> MILDADYITEDGKPVIRVFKKEKGEFKIDYDRDFEPYIYALLKDDSAIEDIKKITAERHGTTVRVTRAERVKKKFLGRPVEVWKLYFTHPQDVPAIRDKIREHPAVVDIYEYDIPFAKRYLIDRGLIPMEGDEELRMLAFDIETLAHAGAAAGAGPILMISYADEEGARVITWKNIDLPYVESVSTEKEMIKRFLKVIQEKDPDVLITYNGDNFDFAYLKKRSEMLGVKFILGRDGSEPKIQRMGDRFAVEVKGRIHFDLYPVIRRTINL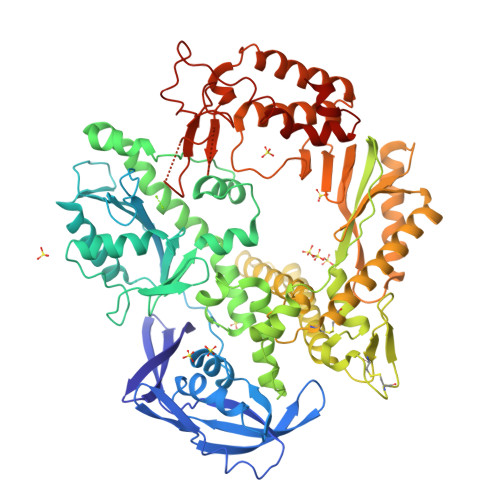PTYTLETVYEPVFGQPAEKVYAEEIAEAWASGEGLERVARYSMEDAKATYELGKEFFPMEAQLSRLVGQSLWDVSRSSTGNLVEWFLLRKAYERNDVAPNKPDERELARRTESYAGGYVKEPEKGLWENIVYLDYKSLYPSIIITHNVSPDTLNREGCREYDVAPQVGHRFCKDFPGFIPSLLGDLLEERQKVKKKMKATVDPIERKLLDYRQRAIKILANSYYGYYAYANARWYCRECAESVTAWGRQYIETTMREIEEKFGFKVLYADTDGFFATIPGADAETVKNKAKEFLNYINPRLPGLLELEYEGFYRRGFFVTKKKYAVIDEEDKITTRGLEIVRRDWSEIAKETQARVLEAILKHGDVEEAVRIVKEVTEKLSRHEVPPEKLVIYEAGPHVAAAATVISYIVLKGPGRVGDRAIPFDEFDPAKHRYDAEYYIENQVLPAVERILRAFGYRKEDLR> DRSANTNIAVYWGQNSAGTQESLATYCESSDADIFLLSFLNQFPTLGLNFANACSDTFSDGLLHCTQIAEDIETCQSLGKKVLLSLGGASGSYLFSDDSQAETFAQTLWDTFGEGTGASERPFDSAVVDGFDFDIENNNEVGYSALATKLRTLFAEGTKQYYLSAAPQCPYPDASVGDLLENADIDFAFIQFYNNYCSVSGQFNWDTWLTYAQTVSPNKNIKLFLGLPGSASAAGSGYISDTSLLESTIADIASSSSFGGIALWDASQAFSNELNGEPYV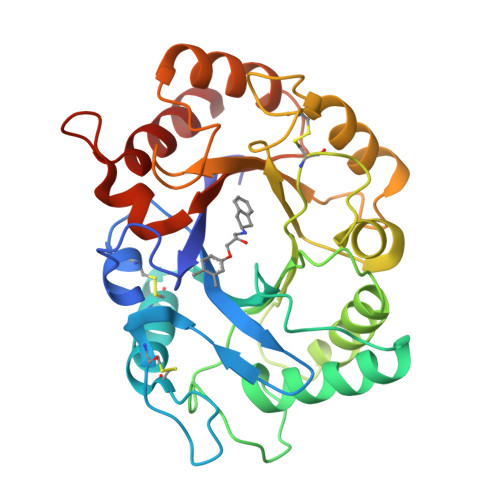EILKNLLTSASQTA>LGTNYLLSGQTLDTEGHLKNGDFDLVMQDDCNLVLYNGNWQSNTANNGRDCKLTLTDYGELVIKNGDGSTVWKSGAQSVKGNYAAVVHPDGRLVVFGPSVFKIDPWVRG[2x];>NIPFTNNLLFSGQVLYGDGRLTAKNHQLVMQGDCNLVLYGGKYGWQSNTHGNGEHCFLRLNHKGELIIKDDDFKTIWSSRSSSKQGEYVLILQDDGFGVIYGPAIFE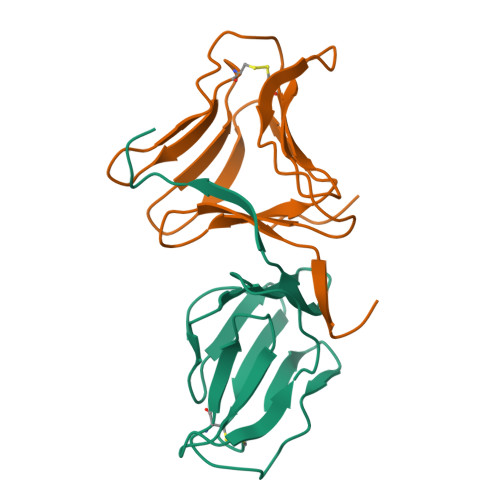TSS[2x]> TG;> CA;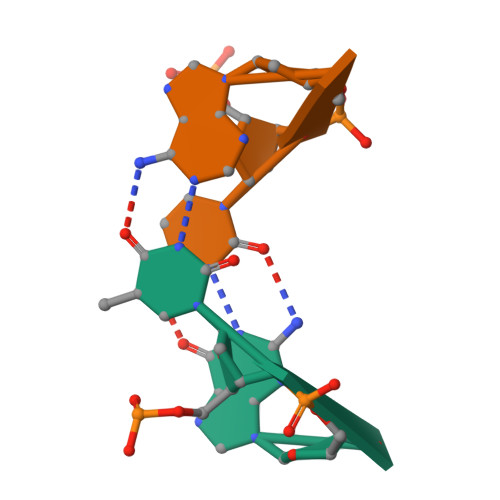> TGTG;> CACA The zinc-dependent metalloprotease meprin α is predominantly expressed in the brush border membrane of proximal tubules in the kidney and enterocytes in the small intestine and colon. In normal tissue homeostasis meprin α performs key roles in inflammation, immunity, and extracellular matrix remodelling. In contrast to meprin β, meprin α is secreted into the extracellular space, whereupon it oligomerises to form giant assemblies and is the largest extracellular protease identified to date (~6 MDa). Here, using cryo-electron microscopy, we determine the high-resolution structure of the zymogen and mature form of meprin α, as well as the structure of the active form in complex with a prototype small molecule inhibitor and human fetuin-B. Our data reveal that meprin α forms a giant, flexible, left-handed helical assembly of roughly 22 nm in diameter.

Unlike small molecule substrates and inhibitors, which are not sterically occluded by the helical packing, we investigated the inhibition of meprin α in vitro by murine fetuin-B, a 42 kDa globular protein. Remarkably, we observed no significant difference in the inhibitory capacity of fetuin-B between oligomeric and monomeric variants of meprin α indicating the oligomer does not interfere with binding. Molecular docking analysis of fetuin-B to the meprin α oligomer instead suggests a compact, intercalated packing is possible that is not impacted by the helical rise of meprin α. We therefore imaged meprin α in complex with human fetuin-B by cryo-EM and generated a 3.7 Å resolution reconstruction. Indeed, this structure confirms the intricate packing suggested by the molecular docking analysis, albeit with some degree of flexibility. The presence of a conserved interface suggests the oligomeric nature of meprin α confers a selection pressure on fetuin-B and supports the notion that meprin α oligomers exist in vivo. Indeed, structural studies of human fetuin-B in complex with meprin α are consistent with crystal structures of murine fetuin-B and meprin β73. Unlike meprin β, these inhibitory complexes were observed to form supramolecular helical packing as a result of the intercalated arrangement of meprin α and numerous fetuin-B molecules.

>[2x]MGLLLPLALCILVLCCGAMSPPQLALNPSALLSRGCNDSDVLAVAGFALRDINKDRKDGYVLRLNRVNDAQEYRRGGLGSLFYLTLDVLETDCHVLRKKAWQDCGMRIFFESVYGQCKAIFYMNNPSRVLYLAAYNCTLRPVSKKKIYMTCPDCPSSIPTDSSNHQVLEAATESLAKYNNENTSKQYSLFKVTRASSQWVVGPSYFVEYLIKESPCTKSQASSCSLQSSDSVPVGLCKGSLTRTHWEKFVSVTCDFFESQAPATGSENSAVNQKPTNLPKVEESQQKNTPPTDSPSKAGPRGSVQYLPDLDDKNSQEKGPQEAFPVHLDLTTNPQGETLDISFLFLEPMEEKLVVLPFPKEKARTAECPGPAQNASPLVLPPHHHHHH;>WSHPQFEKVPIKYLPEENVHDADFGEQKDISEINLAAGLDLFQGDILLQKSRNGLRDPNTRWTFPIPYILADNLGLNAKGAILYAFEMFRLKSCVDFKPYEGESSYIIFQQFDGCWSEVGDQHVGQNISIGQGCAYKAIIEHEILHALGFYHEQSRTDRDDYVNIWWDQILSGYQHNFDTYDDSLITDLNTPYDYESLMHYQPFSFNKNASVPTITAKIPEFNSIIGQRLDFSAIDLERLNRMYNCTTTHTLLDHCTFEKANICGMIQGTRDDTDWAHQDSAQAGEVDHTLLGQCTGAGYFMQFSTSSGSAEEAALLESRILYPKRKQQCLQFFYKMTGSPSDRLVVWVRRDDSTGNVRKLVKVQTFQGDDDHNWKIAHVVLKEEQKFRYLFQGTKGDPQNSTGGIYLDDITLTETPCPTGVWTVRNFSQVLENTSKGDKLQSPRFYNSEGYGFGVTLYPNSRESSGYLRLAFHVCSGENDAILEWPVENRQVIITILDQEPDVRNRMSSSMVFTTSKSHTSPAINDTVIWDRPSRVGTYHTDCNCFRSIDLGWSGFISHQMLKRRSFLKNDDLIIFVDFEDITHLS[4x]> DTCGSGYNVDQRRTNSGCKAGN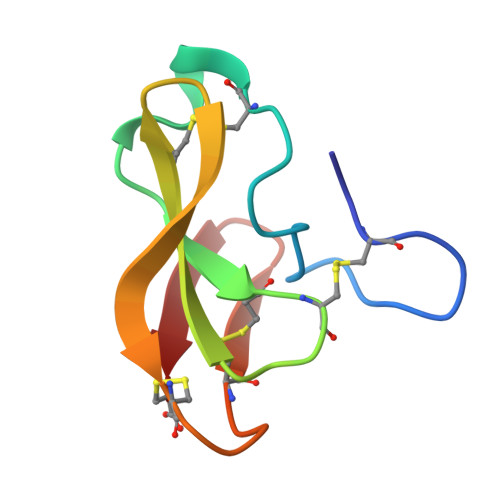GDRHFCGCDRTGVVECKGGKWTEVQDCGSSSCKGTSNGGATC>MAAHRPVEWVQAVVSRFDEQLPIKTGQQNTHTKVSTEHNKECLINISKYKFSLVISGLTTILKNVNNMRIFGEAAEKNLYLSQLIILDTLEKCLAGQPKDTMRLDETMLVKQLLPEICHFLHTCREGNQHAAELRNSASGVLFSLSCNNFNAVFSRISTRLQELTVCSEDNVDVHDIELLQYINVDCAKLKRLLKETAFKFKALKKVAQLAVINSLEKAFWNWVENYPDEFTKLYQIPQTDMAECAEKLFDLVDGFAESTKRKAAVWPLQIILLILCPEIIQDISKDVVDENNMNKKLFLDSLRKALAGHGGSRQLTESAAIACVKLCKASTYINWEDNSVIFLLVQSMVVDLKNLLFNPSKPFSRGSQPADVDLMIDCLVSCFRISPHNNQHFKICLAQNSPSTFHYVLVNSLHRIITNSALDWWPKIDAVYCHSVELRNMFGETLHKAVQGCGAHPAIRMAPSLTFKEKVTSLKFKEKPTDLETRSYKYLLLSMVKLIHADPKLLLCNPRKQGPETQGSTAELITGLVQLVPQSHMPEIAQEAMEALLVLHQLDSIDLWNPDAPVETFWEISSQMLFYICKKLTSHQMLSSTEILKWLREILICRNKFLLKNKQADRSSCHFLLFYGVGCDIPSSGNTSQMSMDHEELLRTPGASLRKGKGNSSMDSAAGCSGTPPICRQAQTKLEVALYMFLWNPDTEAVLVAMSCFRHLCEEADIRCGVDEVSVHNLLPNYNTFMEFASVSNMMSTGRAALQKRVMALLRRIEHPTAGNTEAWEDTHAKWEQATKLILNYPKAKMEDGQAAESLHKTIVKRRMSHVSGGGSIDLSDTDSLQEWINMTGFLCALGGVCLQQRSNSGLATYSPPMGPVSERKGSMISVMSSEGNADTPVSKFMDRLLSLMVCNHEKVGLQIRTNVKDLVGLELSPALYPMLFNKLKNTISKFFDSQGQVLLTDTNTQFVEQTIAIMKNLLDNHTEGSSEHLGQASIETMMLNLVRYVRVLGNMVHAIQIKTKLCQLVEVMMARRDDLSFCQEMKFRNKMVEYLTDWVMGTSNQAADDDVKCLTRDLDQASMEAVVSLLAGLPLQPEEGDGVELMEAKSQLFLKYFTLFMNLLNDCSEVEDESAQTGGRKRGMSRRLASLRHCTVLAMSNLLNANVDSGLMHSIGLGYHKDLQTRATFMEVLTKILQQGTEFDTLAETVLADRFERLVELVTMMGDQGELPIAMALANVVPCSQWDELARVLVTLFDSRHLLYQLLWNMFSKEVELADSMQTLFRGNSLASKIMTFCFKVYGATYLQKLLDPLLRIVITSSDWQHVSFEVDPTRLEPSESLEENQRNLLQMTEKFFHAIISSSSEFPPQLRSVCHCLYQATCHSLLNKATVKEKKENKKSVVSQRFPQNSIGAVGSAMFLRFINPAIVSPYEAGILDKKPPPRIERGLKLMSKILQSIANHVLFTKEEHMRPFNDFVKSNFDAARRFFLDIASDCPTSDAVNHSLSFISDGNVLALHRLLWNNQEKIGQYLSSNRDHKAVGRRPFDKMATLLAYLGPPEHKPVADTHWSSLNLTSSKFEEFMTRHQVHEKEEFKALKTLSIFYQAGTSKAGNPIFYYVARRFKTGQINGDLLIYHVLLTLKPYYAKPYEIVVDLTHTGPSNRFKTDFLSKWFVVFPGFAYDNVSAVYIYNCNSWVREYTKYHERLLTGLKGSKRLVFIDCPGKLAEHIEHEQQKLPAATLALEEDLKVFHNALKLAHKDTKVSIKVGSTAVQVTSAERTKVLGQSVFLNDIYYASEIEEICLVDENQFTLTIANQGTPLTFMHQECEAIVQSIIHIRTRWELSQPDSIPQHTKIRPKDVPGTLLNIALLNLGSSDPSLRSAAYNLLCALTCTFNLKIEGQLLETSGLCIPANNTLFIVSISKTLAANEPHLTLEFLEECISGFSKSSIELKHLCLEYMTPWLSNLVRFCKHNDDAKRQRVTAILDKLITMTINEKQMYPSIQAKIWGSLGQITDLLDVVLDSFIKTSATGGLGSIKAEVMADTAVALASGNVKLVSSKVIGRMCKIIDKTCLSPTPTLEQHLMWDDIAILARYMLMLSFNNSLDVAAHLPYLFHVVTFLVATGPLSLRASTHGLVINIIHSLCTCSQLHFSEETKQVLRLSLTEFSLPKFYLLFGISKVKSAAVIAFRSSYRDRSFSPGSYERETFALTSLETVTEALLEIMEACMRDIPTCKWLDQWTELAQRFAFQYNPSLQPRALVVFGCISKRVSHGQIKQIIRILSKALESCLKGPDTYNSQVLIEATVIALTKLQPLLNKDSPLHKALFWVAVAVLQLDEVNLYSAGTALLEQNLHTLDSLRIFNDKSPEEVFMAIRNPLEWHCKQMDHFVGLNFNSNFNFALVGHLLKGYRHPSPAIVARTVRILHTLLTLVNKHRNCDKFEVNTQSVAYLAALLTVSEEVRSRCSLKHRKSLLLTDISMENVPMDTYPIHHGDPSYRTLKETQPWSSPKGSEGYLAATYPTVGQTSPRARKSMSLDMGQPSQANTKKLLGTRKSFDHLISDTKAPKRQEMESGITTPPKMRRVAETDYEMETQRISSSQQHPHLRKVSVSESNVLLDEEVLTDPKIQALLLTVLATLVKYTTDEFDQRILYEYLAEASVVFPKVFPVVHNLLDSKINTLLSLCQDPNLLNPIHGIVQSVVYHEESPPQYQTSYLQSFGFNGLWRFAGPFSKQTQIPDYAELIVKFLDALIDTYLPGIDEETSEESLLTPTSPYPP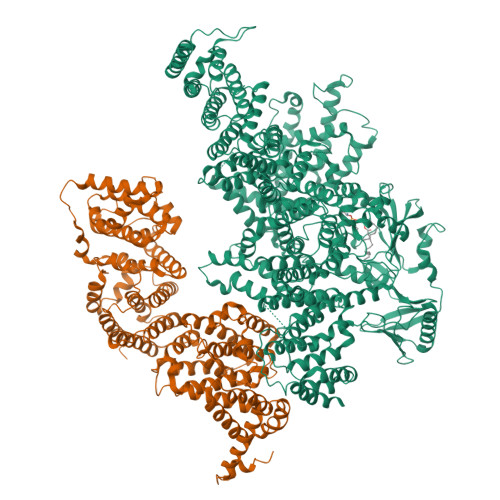ALQSQLSITANLNLSNSMTSLATSQHSPGIDKENVELSPTTGHCNSGRTRHGSASQVQKQRSAGSFKRNSIKKIV[2x]(2S)-(3-{[AMINO(IMINO)METHYL]AMINO}PHENYL){[(S)-HYDROXY{(1R)-2-METHYL-1-[(3-PHENYLPROPANOYL)AMINO]PROPYL}PHOSPHORYL]OXY}ACETIC 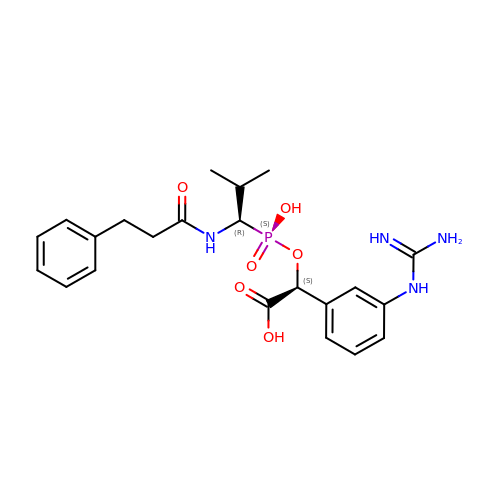ACID | C22 H29 N4 O6 P | FCWKSOJGKKFIAW-VQTJNVASSA-N> MQRVVVAIDAKRVDGEFMVFTHSGKKNTGILLRDWVVEVEKRGAGEILLTSIDRDGTKSGYDTEMIRFVRPLTTLPIIASGGAGKMEHFL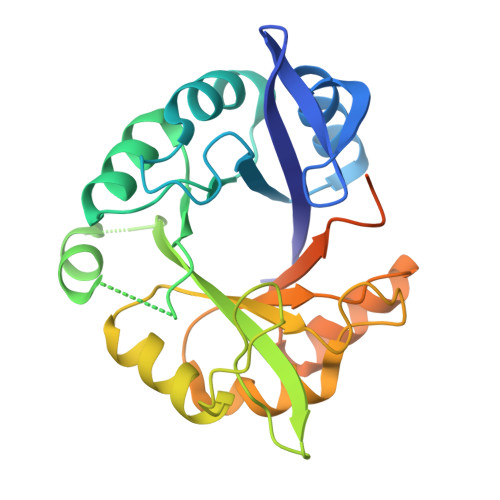EAFLAGADKALAASVFHFREIDMRELKEYLKKHGGSGQAVVVAIDAKRVDGEFMVFTHSGKKNTGILLRDWVVEVEKRGAGEILLTSIDRDGTKSGYDTEMIRFVRPLTTLPIIASGGAGKMEHFLEAFLAGADAALAASVFHFREIDMRELKEYLKKHGVNVRLEGLLEHHHHHH>[2x]HDPLTGLPNRRYFFELGNRYLDLAKRE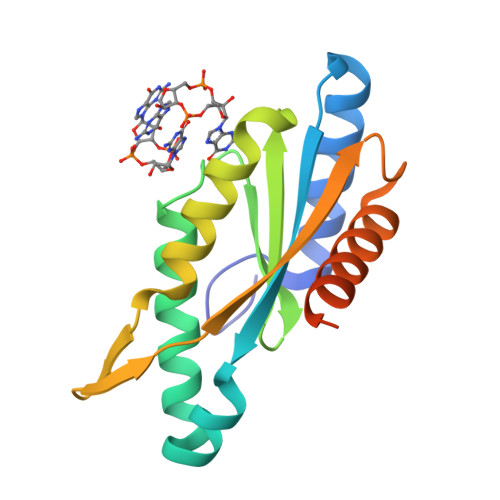GKKVFVLFVDLAGFKAINDTYGHLSGDEVLKTVSKRILDRVRRSDVVARYGGDEFTILLYDMKEEYLKSLLERILSTFREPVRVENKHLSVTPNIGVARFPEDGENLEELLKVADMRMYKAKEMKVPYFSLSLEHHHHHH> VKDTYTDRLDDWNGIIAGNQYYDSKNDQMAKLNQELEGKVADSLSSISSQADRIYLWEKFSNYKTSANLTATYRKLEEMAKQVTNPSSRYYQDETVVRTVRDSMEWMHKHVYNSEKSIVGNWADYEIGTPRAINNTLSLMKEYFSDEEIKKYTDVIEKFVPDPEHFRKTTDNPVKALGGNLVDMGRVKVIAGLLRKDDQEISSTIRSIEQVFKLVDQGEGFYQDGSYIDHTNVAYTGAYGNVLIDGLSQLLPVIQKTKNPIDKDKMQTMYHWIDKSFAPLLVNGELMDMSRGRSISRANSEG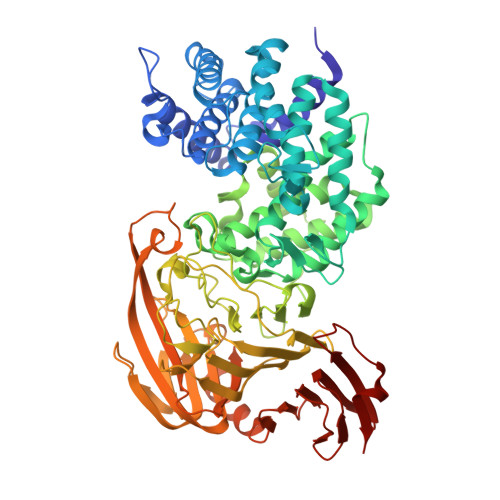HVAAVEVLRGIHRIADMSEGETKQRLQSLVKTIVQSDSYYDVFKNLKTYKDISLMQSLLSDAGVASVPRTSYLSAFNKMDKTAMYNAEKGFGFGLSLFSSRTLNYEHMNKENKRGWYTSDGMFYLYNGDLSHYSDGYWPTVNPYKMPGTTETDAKRADSDTGKVLPSAFVGTSKLDDANATATMDFTNWNQTLTAHKSWFMLKDKIAFLGSNIQNTSTDTAATTIDQRKLESSNPYKVYVNDKEASLTEQEKDYPETQSVFLESSDSKKNIGYFFFKKSSISMSKALQKGAWKDINEGQSDKEVENEFLTISQAHKQNGDSYGYMLIPNVDRATFNQMIKELESSLIENNETLQSVYDAKQGVWGIVKYDDSVSTISNQFQVLKRGVYTIRKEGDEYKIAYYNPETQESAPDQEVFKKL>[2x]MGSSHHHHHHENLYFQGMKFTVIAKAIFILGILTTSVMITENQSVNAKGKYEKMNRLYDTNKLHQYYSGPSYELTNVSGQSQGYYDSNVLLFNQQN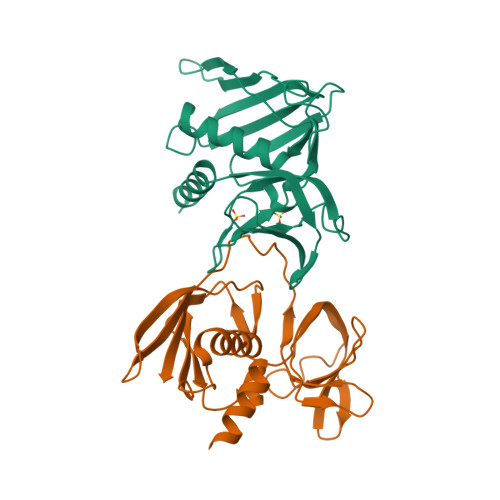QKFQVFLLGKDENKYKEKTHGLDVFAVPELVDLDGRIFSVSGVTKKNVKSIFESLRTPNLLVKKIDDKDGFSIDEFFFIQKEEVSLKELDFKIRKLLIKKYKLYEGSADKGRIVINMKDENKYEIDLSDKLDFERMADVINSEQIKNIEVNLK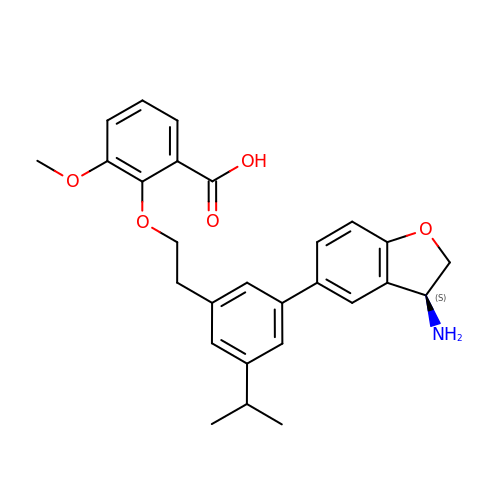2-[2-[3-[(3~{S})-3-azanyl-2,3-dihydro-1-benzofuran-5-yl]-5-propan-2-yl-phenyl]ethoxy]-3-methoxy-benzoic acid | C27 H29 N O5 | KXSZMPGKDDBJRE-HSZRJFAPSA-N> MSGNPASSSEQNNNSYETKASLRISEKKCSWASYMTNSPTLIVMIGLPARGKTYVSKKLTRYLNWIGVPTKVFNLGVYRRQAVKSYKSYDFFRHDNEEAMKIRKQCALVALKDVKAYLTEESGQIAVFDATNTTRERRDLILNFAEENSFKVFFVESVCDDPDVIAANILEVKVSSPDYPERNRENVMDDFLKRIECYKVTYQPLDPDSHDKDLSFIKVINVGQRFLVNKVQDYIQSKIVYYLMNIHVHPRTIYLCRHGESEFNLLGKIGGDSGLSVRGKQFAQALRKFLEEQEIADLKVWTSQLKRTIQTAESLGVTYEQWKILNEIDAGVCEEMTYAEIQEQYPDEFALRDEEKYLYRYPGGESYQDLVQRLEPVIMELERQGNVLVISHQAVMRCLLAYFLDKGADELPYLRCPLHTIFK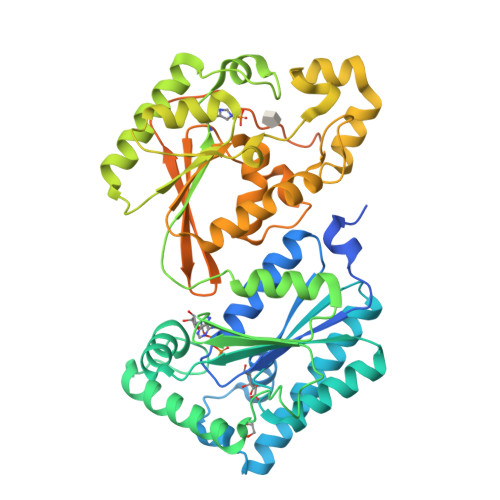LTPVAYGCKVETIKLNVEAVNTHRDKPTNNFPKNQTPVRMRRNSFTPLSSSNTIRRPRNYSVGSRPLQPLSPLRALDTQEGADQPKTQAETSRAAHRLPSPAPPTSPS> SNAMKISDA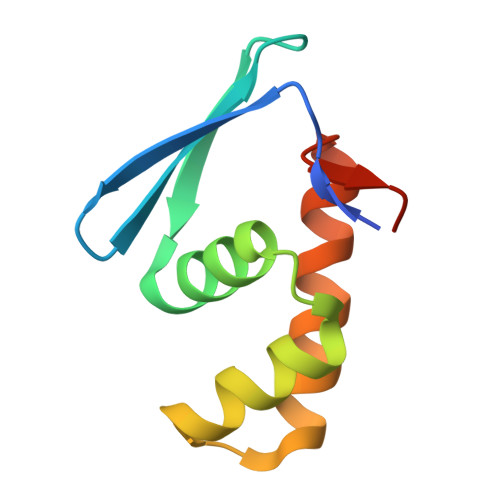VVSAHIDDEVVLLHLQTGTYFGLDAVGSRIWSLLEEGKRPEEIVDAICAEYSVDRPTVERDLRDFLRALANKELLEGYADEA>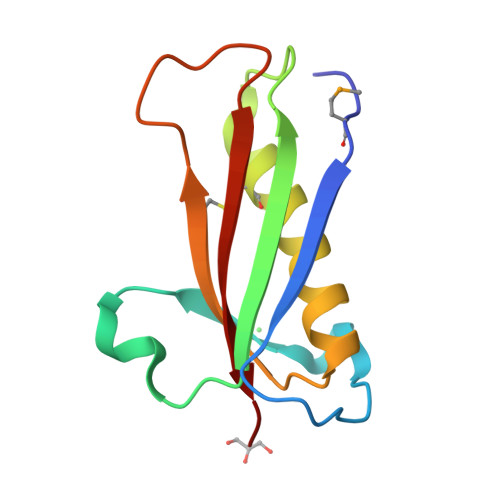 GSHMETKGVYLPKYSAELPPTDPSQVRVYNLQYQSDTQGNIGQVRTSTHVSNEKDFQKLCDKNLKEAIKLAAQHGAHEIKYICLYPEGQINELSSVQLRGYAFRD> AKPGPALWPLPLSVKMTPNLLHLAPENFYISHSPNSTAGPSCTLLEEAFRRYHGYIFGFYKWHHEPAEFQAKTQVQQLLVSITLQSECDAFPNISSDESYTLLVKEPVAVLKANRVWGALRGLETFSQLVYQDSYGTFTINESTIIDSPRFSHRGILIDTSRHYLPVKI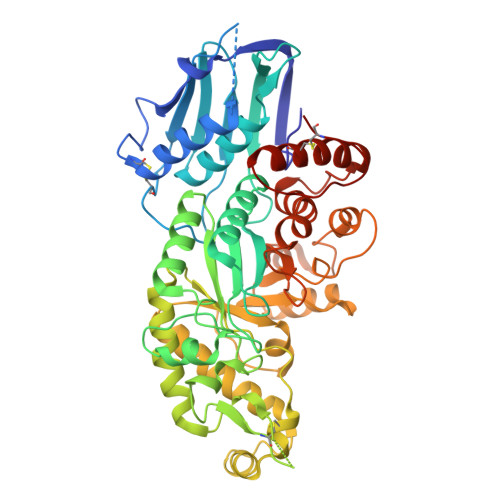ILKTLDAMAFNKFNVLHWHIVDDQSFPYQSITFPELSNKGSYSLSHVYTPNDVRMVIEYARLRGIRVLPEFDTPGHTLSWGKGQKDLLTPCYSRQNKLDSFGPINPTLNTTYSFLTTFFKEISEVFPDQFIHLGGDEVEFKCWESNPKIQDFMRQKGFGTDFKKLESFYIQKVLDIIATINKGSIVWQEVFDDKAKLAPGTIVEVWKDSAYPEELSRVTASGFPVILSAPWYLDLISYGQDWRKYYKVEPLDFGGTQKQKQLFIGGEACLWGEYVDATNLTPRLWPRASAVGERLWSSKDVRDMDDAYDRLTRHRCRMVERGIAAQPLYAGYCNHENM The REV-ERBs, REV-ERBα (NR1D1) and REV-ERBβ (NR1D2), are closely related NRs with critical roles in mammalian physiology, including maintenance of the circadian rhythm, metabolic processes, and immune function. The REV-ERBs are unique among NRs because their ligand-binding domains (LBDs) lack the C-terminal activation function–2 (AF-2) helix 12 important for binding transcriptional coactivator proteins, suggesting that the REV-ERBs should interact exclusively with transcriptional corepressor proteins and solely repress transcription. The iron-centered porphyrin heme has been identified as the endogenous REV-ERB ligand. REV-ERB LBD interacts with NCoR via two ID motifs present within the RID.

Using two fluorescence-independent methods, isothermal titration calorimetry (ITC) and nuclear magnetic resonance (NMR) spectroscopy, we show that heme directly increases REV-ERBβ LBD affinity for one of two ID motif peptides within the NCoR receptor ID (RID). Heme decreased LBD affinity for the ID1 peptide but increased LBD affinity for ID2 peptide, effectively equalizing the ID1 and ID2 peptide affinities. Titration of both peptides into heme-bound LBD revealed a mixture of peak movements in slow and intermediate exchange, consistent with the moderate affinities (~2 μM) of these interactions measured by ITC. To determine the structural basis of this interaction, we solved crystal structures of REV-ERBβ LBD cobound to heme and NCoR ID1 peptide (2.6-Å resolution) or ID2 peptide (2.0-Å resolution) (respectively). In both structures, REV-ERBβ LBD crystallized with two molecules in the asymmetric unit with an NCoR ID peptide and heme molecule cobound to each LBD. The overall root mean square deviation (RMSD) of the complex in the asymmetric unit including LBD, heme, and NCoR ID peptide was 1.1 and 1.3 Å for the ID1- and ID2-bound structures, respectively, suggesting minimal conformational heterogeneity. The ID peptides bound to the AF-2 surface formed electrostatic interactions with the conserved charge clamp residue K421 on helix 3, confirming that the heme-dependent REV-ERBβ corepressor interaction is similar to other NRs. The overall heme-bound LBD conformations were largely unchanged by peptide binding, with average LBD RMSDs of 1.0 and 1.3 Å for the ID1- and ID2-bound structures, respectively, relative to the published heme-bound LBD structure.

>[2x]HLVCPMSKSPYVDPHKSGHEIWEEFSMSFTPAVKEVVEFAKRIPGFRDLSQHDQVNLLKAGTFEVLMVRFASLFDAKERTVTFLSGKKYSVDDLHSMGAGDLLNSMFEFSEKLNALQLSDEEMSLFTAVVLVSADRSGIENVNSVEALQETLIRALRTLIMKNHPNEASIFTKLLLKLPDLRSLNNMHSEELLAFKVHP;>[2x]DPASNLGLEDIIRKALMGSFDDK> MVAESNSAVAPTANVATSPAHEHFVRVNGGHFELQGKPYVITGVNMWYAAYLGAPNEVGDRDRLAKELDNLKAIGVNNLRVLAVSEKSEINSAVKPAVTNGFGNYDETLLQGLDYLLVELAKRDMTVVLYFNNFWQWSGGMTQYMAWIEGEPVQDPNVTNEWEAFMAKSASFYRSEKAQQEYRKTLEKIITRVNSINGKAYVDDATIMSWQLANEPRPGNSQTTAEEKQIYIDWVHAAAAYIKTLDAHHLVSSGSEGEMGSVNDMQVFIDAHATPDIDYLTYHMWIRNWSWFDKTKPAETWPSAWEKAQNYMRAHIDVAKQLNKPLVLEEFGLDRDMGSYAMDSTTEYRDNYFRGVFELMLASLEQGEPSAGYNIWAWNGYGRTTRANYWWQEGDDFMGDPPQEEQGMYGVFDTDTSTIAIMKEFNARFQPKLEHHHHHH

Exo-β-mannosidases, hydrolysing non-reducing terminal β-d-mannopyranosidic linkages, are widely distributed carbohydrate-degrading enzymes. All of these exo-β-mannosidases process their substrate using a stereochemically retaining double displacement mechanism that is characterised by the formation of a covalent glycosyl enzyme intermediate (GEI). We show that these probes covalently label exo-β-mannosidases from GH families 2, 5, and 164. Structural studies of the resulting complexes support a canonical mechanism-based mode of action in which the active site nucleophile attacks the pseudoanomeric centre to form a stable ester linkage, mimicking the glycosyl enzyme intermediate.

CmMan5A showed 20% inhibition with both 1 and 2, and stronger 85% inhibition with 3, indicating that binding is enhanced by the presence of the alkyl group. CmMan5A bound to compound 3 gave the highest resolution structure at 1.3 Å. Supporting our hypothesized mechanism of reactivity, compound 3 was covalently linked to E330, the known catalytic nucleophile, through its pseudoanomeric carbon. The ring was found in an OS2-like conformation, providing the first direct evidence that the GEI conformation for GH5 β-mannosidases matches that of GH2 β-mannosidases and GH26 β-mannanases. The amine group from the opened aziridine is found interacting with both the general acid, E215, and an apparent buffer acetate that also interacts with the axial O3. C7 (taking the place of endocyclic oxygen) forms a CH/π interaction (3.4 Å) with W285 while the alkyl chain extends out of the catalytic pocket, forming hydrophobic packing interactions with W285, W135, and a hydrophobic groove between N288 and W289. We speculate that these interactions contribute to the observed tighter binding of compound 3 over compound 2. Indeed, the first four carbons of the alkyl linker display well-localised electron density (B factors of 16–25 Å2), indicating rigid binding and suggesting that a shorter linker may hinder binding into the active site pocket.> NAAYYQVVPVTANVYDSDGEKLSYISQGSVVWLDKDRKSDDKRLAITISGLSGYMKTEDLQALDASKDFIPYYESDGHRFYHYVAQNASIPVASHLSDMEVGKKYYSADGLHFDGFKLENPFLFKDLTEATNYSAEELDKVFSLLNINNSLLENKGATFKEAEEHYHINALYLLAHSALESNWGRSKIAKDKNNFFGITAYDTTPYLSAKTFDDVDKGILGATKWIKEN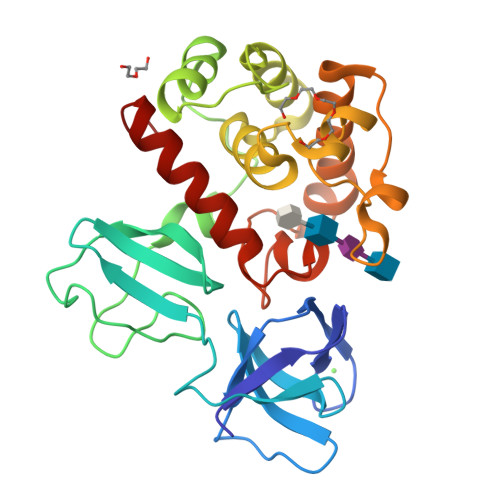YIDRGRTFLGNKASGMNVEYASDPYWGEKIASVMMKINEKLGGKD> GRPANANSGFYVSGTTLYDANGNPFVMRGINHGHAWYKDQATTAIEGIANTGANTVRIVLSDGGQWTKDDIQTVRNLISLAEDNNLVAVLEVHDATGYDSIASLNRAVDYWIEMRSALIGKEDTVIINIANEWFGSWDGAAWADGYKQAIPRLRNAGLNNTLMIDAAGWGQF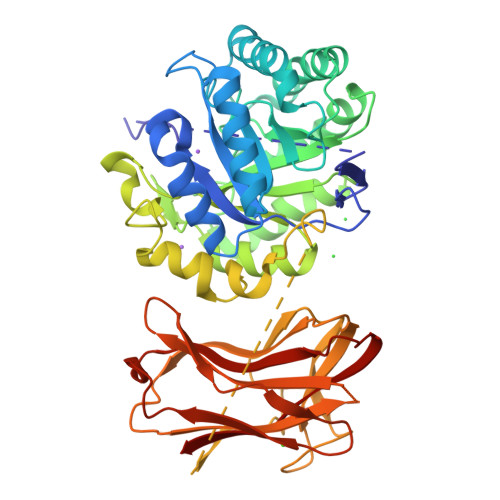PQSIHDYGREVFNADPQRNTMFSIHMYEYAGGNASQVRTNIDRVLNQDLALVIGEFGHRHTNGDVDESTIMSYSEQRGVGWLAWSWKGNGPEWEYLDLSNDWAGNNLTAWGNTIVNGPYGLRETSKLSTVFTGGGSDGRTSPTTLYDFEESTQGWTGSSLSRGPWTVTEWSSKGNHSLKADIQMSSNSQHYLHVIQNRSLQQNSRIQATVKHANWGSVGNGMTARLYVKTGHGYTWYSGSFVPINGSSGTTLSLDLSNVQNLSQVREIGVQFQSESNSSGQTSIYIDNVIVE> MGPSLDF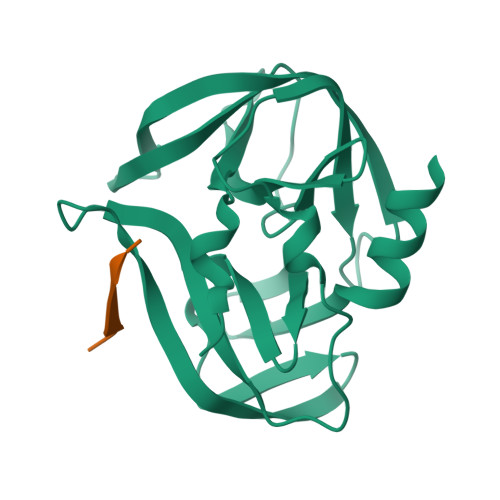ALSLLRRNIRQVQTDQGHFTMLGVRDRLAVLPRHSQPGKTIWIEHKLVNVLDAVELVDEQGVNLELTLITLDTNEKFRDITKFIPENISTASDATLVINTEHMPSMFVPVGDVVQYGFLNLSGKPTHRTMMYNFPTKAGQAGGVVTSVGKVIGIHIGGNGRQGFCAGLKRSYFASEQHHHHHH;> KPVLRTA> MLEKVETFDMNRVIDEFDEMTRNAHQVQKQTLKEILLKNQSAIYLQNCGLNGNATDPEEAFKSMVPLVTDVELEPYIKRMVDGDTSPILTGHPVPAISLSSGTSQGRPKFIPFTDELMENTLQLFRTAFAFRNRDFPIDDNGKALQFIFSSKQYISTGGVPVGTATTNVYRNPNFKAGMKSITSPSCSPDEVIFSPDVHQALYCHLLSGILFRDQVQYVFAVFAHGLVHAFRTFEQVWEEIVTDIKDGVLSNRITVPSVRTAMSKLLTPNPELAETIRTKCMSLSNWYGLIPALFPNAKYVYGIMTGSMEPYVPKLRHYAGDLPLVSHDYGSSEGWIAANVTPRLSPEEATFAVIPNLGYFEFLPVSETGEGEEKPVGLTQVKIGEEYEVVITNYAGLYRYRLGDVVKVIGFYNNTPQLKFICRRNLILSINIDKNTERDLQLSVESAAKRLSEEKIEVIDFSSYIDVSTDPGHYAIFWEISGETNED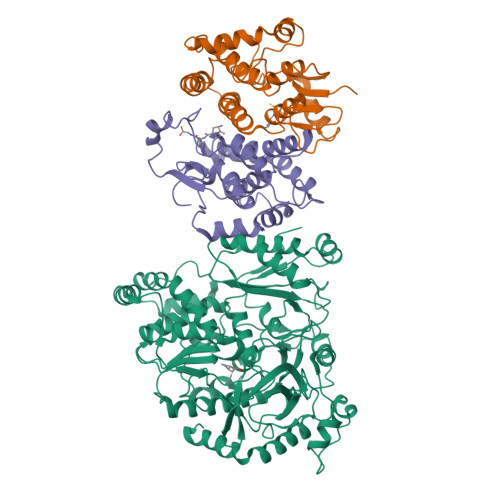VLQDCCNCLDRAFIDAGYVSSRKCKTIGALELRVVAKGTFRKIQEHFLGLGSSAGQFKMPRCVKPSNAKVLQILCENVVSSYFSTAF;>[6x]MSPILGYWKIKGLVQPTRLLLEYLEEKYEEHLYERDEGDKWRNKKFELGLEFPNLPYYIDGDVKLTQSMAIIRYIADKHNMLGGCPKERAEISMLEGAVLDIRYGVSRIAYSKDFETLKVDFLSKLPEMLKMFEDRLCHKTYLNGDHVTHPDFMLYDALDVVLYMDPMCLDAFPKLVCFKKRIEAIPQIDKYLKSSKYIAWPLQGWQATFGGGDHPPK>[2x]FVVRDIRVNGLVRLTPANVYTMLPINSGDRVNEPMIAEAIRTLYATGLFDDIKASKENDTLVFNVIERPIISKLEFKGNKLIPKEALEQGLKKMGIAEGEVFKKSALQTIETELEQQYTQQGRYDADVTVDTVARPNNRVELKINFNEGTPAKVFDINVIGNTVFKDSEI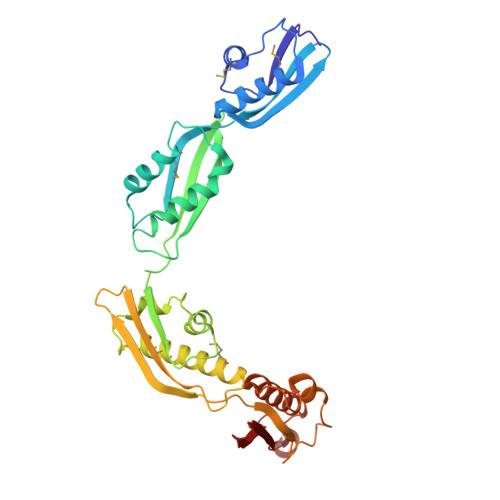KQAFAVKESGWASVVTRNDRYAREKMAASLEALRAMYLNKGYINFNINNSQLNISEDKKHIFIEVAVDEGSQFKFGQTKFLGDALYKPEELQALKIYKDGDTYSQEKVNAVKQLLLRKYGNAGYYFADVNIVPQINNETGVVDLNYYVNPGQQVTVRR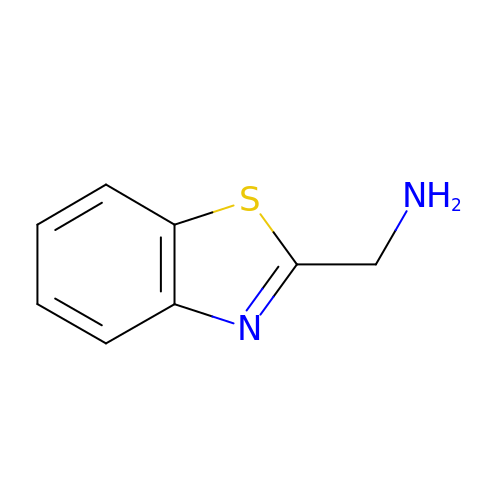1-(1,3-benzothiazol-2-yl)methanamine | C8 H8 N2 S | VLBUERZRFSORRZ-UHFFFAOYSA-N>[2x]MALLPDKEKLLRNFLRCANWEEKYLYIIELGQRLPELRDEDRSPQNSIQGCQSQVWIVMRQNAQGI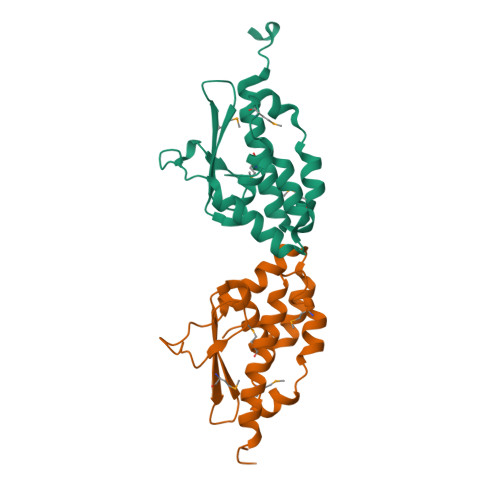IELQGDSDAAIVKGLIAVVFILYDQMTPQDIVNFDVRPWFEKMALTQHLTPSRSQGLEAMIRAIRAKAAALSLEHHHHHH> RPESELIRQSWRVVSRSPLEHGTVLFARLFALEPSLLPLFQYNGRQFSSPEDSLSSPEFLDHIRKVMLVIDAAVTNVEDL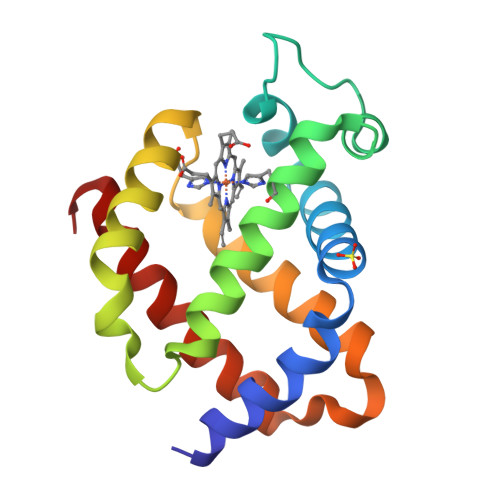SSLEEYLTSLGRKHRAVGVRLSSFSTVGESLLYMLEKSLGPDFTPATRTAWSRLYGAWVQAMSRGWDG> KDRPSLCDLPADSGSGTKAEKRIYYNSARKQCLRFDY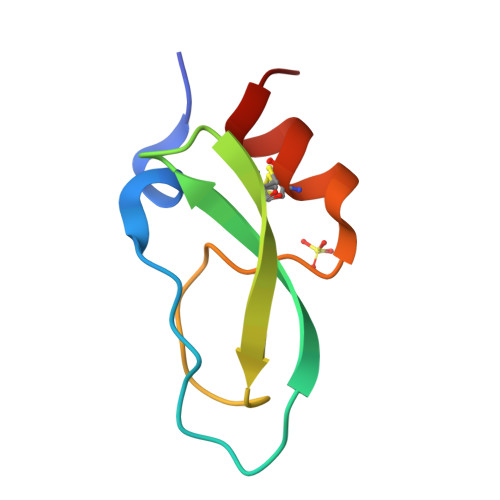TGQGGNENNFRRTYDCARTCLYTA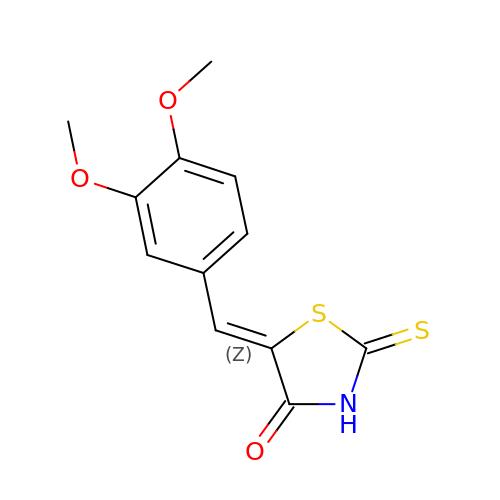(5Z)-5-[(3,4-dimethoxyphenyl)methylidene]-2-sulfanylidene-1,3-thiazolidin-4-one | C12 H11 N O3 S2 | XVAIHVYMCLRIOV-POHAHGRESA-N> MEATLEQRPFPYLATEANLLTQIKESAADGLFKSFQLLLGKDAREGSVRFEALLGVYTNVVEFVKF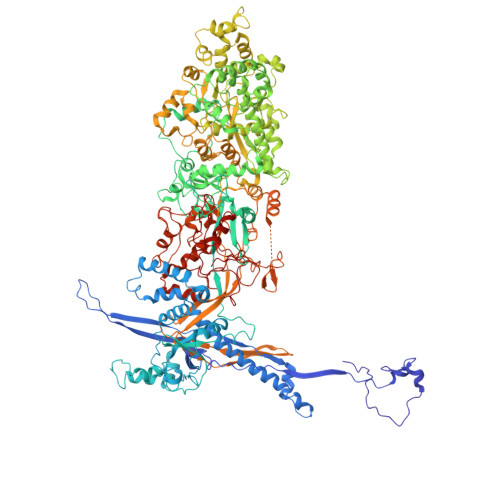LETALAAACVNTEFKDLRRMIDGKIQFKISMPTIAHGDGRRPNKQRQYIVMKACNKHHIGAEIELAAADIELLFAEKETPLDFTEYAGAIKTITSALQFGMDALERGLVDTVLAVKLRHAPPVFILKTLGDPVYSERGLKKAVKSDMVSMFKAHLIEHSFFLDKAELMTRGKQYVLTMLSDMLAAVCEDTVFKGVSTYTTASGQQVAGVLETTDSVMRRLMNLLGQVESAMSGPAAYASYVVRGANLVTAVSYGRAMRNFEQFMARIVDHPNALPSVEGDKAALADGHDEIQRTRIAASLVKIGDKFVAIESLQRMYNETQFPCPLNRRIQYTYFFPVGLHLPVPRYSTSVSVRGVESPAIQSTETWVVNKNNVPLCFGYQNALKSICHPRMHNPTQSAQALNQAFPDPDGGHGYGLRYEQTPNMNLFRTFHQYYMGKNVAFVPDVAQKALVTTEDLLHPTSHRLLRLEVHPFFDFFVHPCPGARGSYRATHRTMVGNIPQPLAPREFQESRGAQFDAVTNMTHVIDQLTIDVIQETAFDPAYPLFCYVIEAMIHGQEEKFVMNMPLIALVIQTYWVNSGKLAFVNSYHMVRFICTHMGNGSIPKEAHGHYRKILGELIALEQALLKLAGHETVGRTPITHLVSALLDPHLLPPFAYHDVFTDLMQKSSRQPIIKIGDQNYDNPQNRATFINLRGRMEDLVNNLVNIYQTRVNEDHDERHVLDVAPLDENDYNPVLEKLFYYVLMPVCSNGHMCGMGVDYQNVALTLTYNGPVFADVVNAQDDILLHLENGTLKDILQAGDIRPTVDMIRVLCTSFLTCPFVTQAARVITKRDPAQSFATHEYGKDVAQTVLVNGFGAFAVADRSREAAETMFYPVPFNKLYADPLVAATLHPLLANYVTRLPNQRNAVVFNVPSNLMAEYEEWHKSPVAAYAASCQATPGAISAMVSMHQKLSAPSFICQAKHRMHPGFAMTVVRTDEVLAEHILYCSRASTSMFVGLPSVVRREVRSDAVTFEITHEIASLHTALGYSSVIAPAHVAAITTDMGVHCQDLFMIFPGDAYQDRQLHDYIKMKAGVQTGPPGNRMDHVGYAAGVPRCENLPGLSHGQLATCEIIPTPVTSDVAYFQTPSNPRGRAACVVSCDAYSNESAERLLYDHSIPDPAYECRSTNNPWASQRGSLGDVLYNITFRQTALPGMYSPCRQFFHKEDIMRYNRGLYTLVNEYSARLAGAPATSTTDLQYVVVNGTDVFLDQPCHMLQEAYPTLAASHRVMLDEYMSNKQTHAPVHMGQYLIEEVAPMKRLLKLGNKVVY>QNFLNDQFVIDSIVSAINPQKGQAMVEIGPGLAALTEPVGERLDQLTVIELDRDLAARLQTHPFLGPKLTIYQQDAMTFNFGELAEKMGQPLRVFGNLPYNISTPLMFHLFSYTDAIADMHFMLQKEVVNRLVAGPNSKAYGRLSVMAQYYCNVIPVLEVPPSAFTPPPKVDSAVVRLVPHATMPHPVKDVRVLSR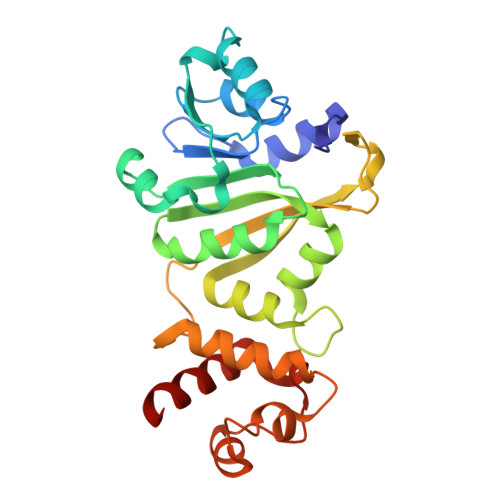ITTEAFNQRRKTIRNSLGNLFSVEVLTGMGIDPAMRAENISVAQYCQMANYLAENA[2x]>RWRAEGTSAHLRDIFLGRCAEYRALLSPEQRNKDCTAIWEAFKVALD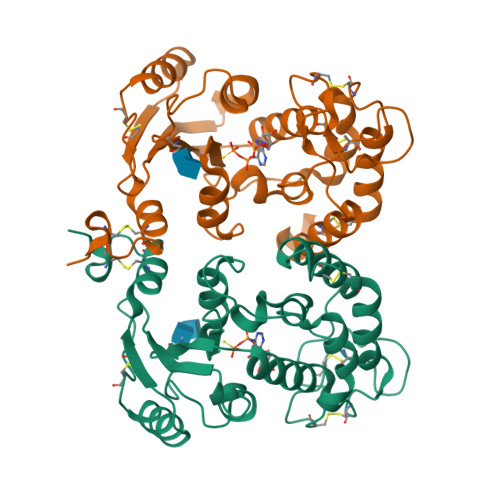KDPCSVLPSDYDLFITLSRHSIPRDKSLFWENSHLLVNSFADNTRRFMPLSDVLYGRVADFLSWCRQKADSGLDYQSCPTSEDCENNPVDSFWKRASIQYSKDSSGVIHVMLNGSEPTGAYPIKGFFADYEIPNLQKEKITRIEIWVMHEIGGPNVESCGEGSMKVLEKRLKDMGFQYSCINDYRPVKLLQCVDHSTHPDCALKSAAAATQRKAPSLY[2x]[6-(3-methoxyphenyl)-2-(4-methoxyphenyl)-1-benzofuran-3-yl]acetic acid | C24 H20 O5 | 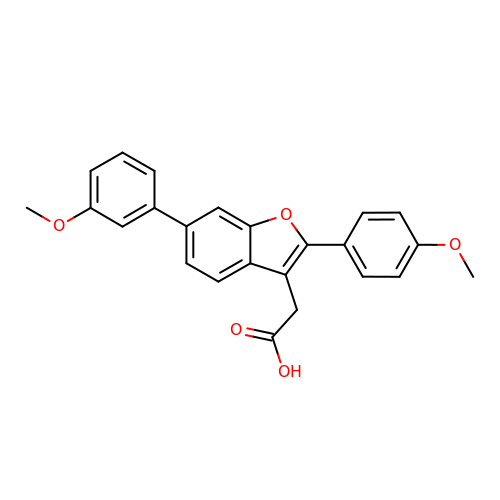TZSONHMMMFCHKL-UHFFFAOYSA-N>[2x]MQVMASPPCTTEELSPPPGGSLVEYSGGSLRVPDNPVVAFIRGDGVGPEVVESALKVVDAAVKKVYGGSRRIVWWELLAGHLAREKCGELLPKATLEGIRLARVALKGPLETPVGTGYRS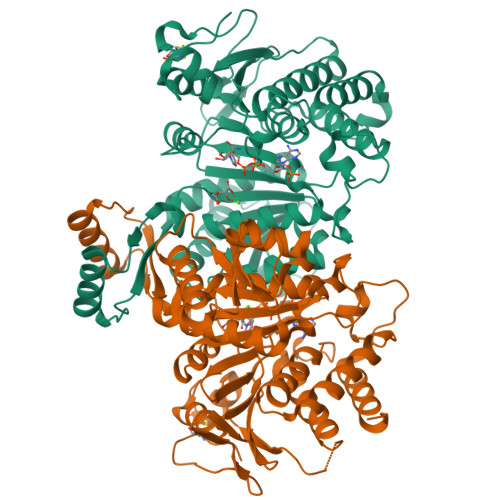LNVAIRQALDLYANIRPVRYYGQPAPHKYADRVDMVIFRENTEDVYAGIEWPHDSPEAARIRRFLAEEFGISIREDAGIGVKPISRFATRRLMERALEWALRNGNTVVTIMHKGNIMKYTEGAFMRWAYEVALEKFREHVVTEQEVQEKYGGVRPEGKILVNDRIADNMLQQIITRPWDYQVIVAPNLNGDYISDAASALVGGIGMAAGMNMGDGIAVAEPVHGTAPKYAGKDLINPSAEILSASLLIGEFMGWREVKSIVEYAIRKAVQSKKVTQDLARHMPGVQPLRTSEYTETLIAYIDEADLNEVLAGKRG> QGGAAAPISSHCRLDKSNFQ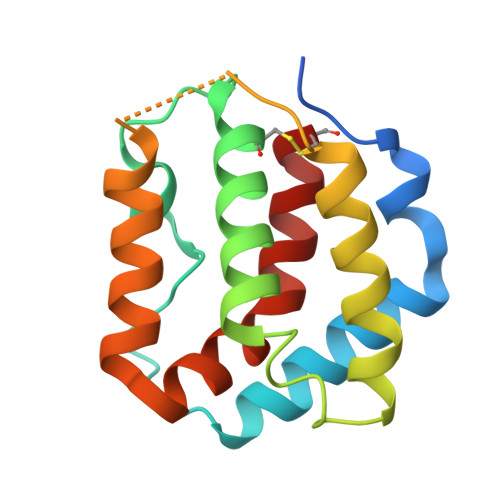QPYITNRTFMLAKEASLADNNTDVRLIGEKLFHGVSMSERCYLMKQVLNFTLEEVLFPQSDRFQPYMQEVVPFLARLSNRLSTCHIEGDDLHIQRNVQKLKDTVKKLGESGEIKAIGELDLLFMSLRNACI> MNLLTMMAATSLPNYLAGNGDLGSWEP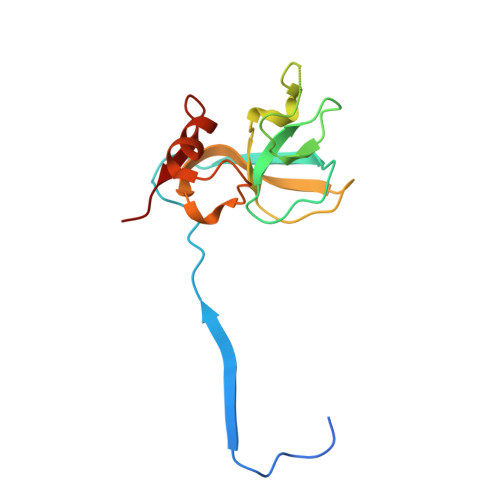TQIFAGEADIVTEGGAAGADIEIYQVIAKNAAGAMVPHDPTATTGTSPDEVPAPQSVAIGIAAQPAKSGQNVPYYIGGVFNHAALGWHASLDTLAKRQAVFDRTNIHIGNLY3-[2-[[5-[(4-ethenyl-3-methyl-5-oxidanylidene-pyrrol-2-yl)methyl]-3-(3-hydroxy-3-oxopropyl)-4-methyl-1~{H}-pyrrol-2-yl]methyl]-5-[[(3~{S})-4-ethyl-3-methyl-2-oxidanylidene-1,3-dihydropyrrol-5-yl]methyl]-4-methyl-1~{H}-pyrrol-3-yl]propanoic 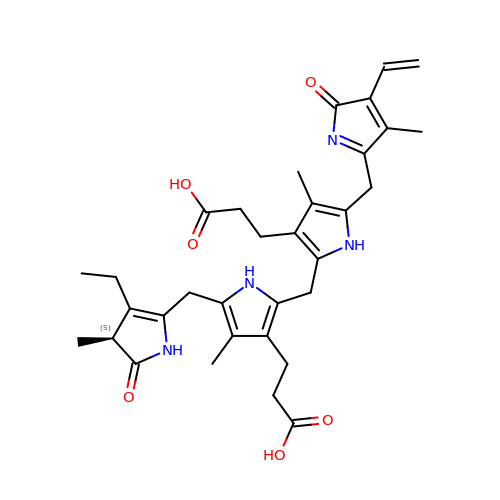acid | C33 H40 N4 O6 | HLNBFSQHDRNIJH-IBGZPJMESA-N octyl 3-amino-3-deoxy-2-O-(2,6-dideoxy-alpha-L-lyxo-hexopyranosyl)-beta-D-galactopyranoside | C20 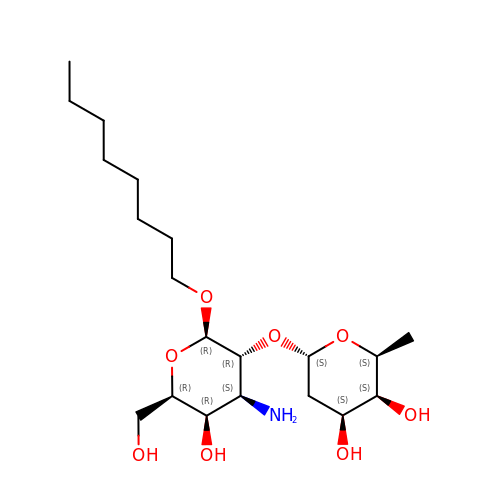H39 N O8 | GHTLMVRROQXELT-HTYYFBMYSA-N>[4x]M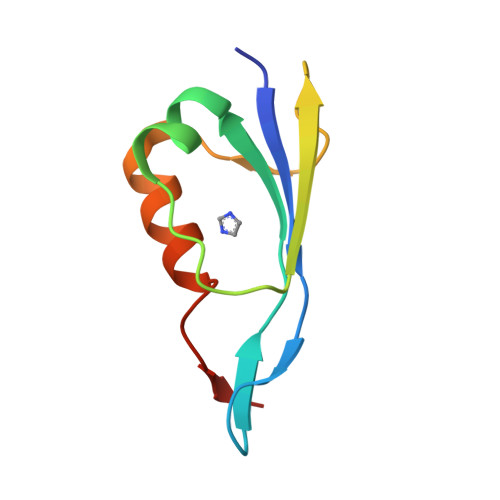GGYVNIKTFTHPAGEGKEVKGMEVSVPFEIYSNEHRIADAHYQTFPSEKAAYTTVVTDAADWRTKNAAMFTPTPVSG2-(2,6-difluorophenyl)-N-(2,6-dimethylphenyl)-5-methylimidazo[1,2-a]pyridin-3-amine | C22 H19 F2 N3 | 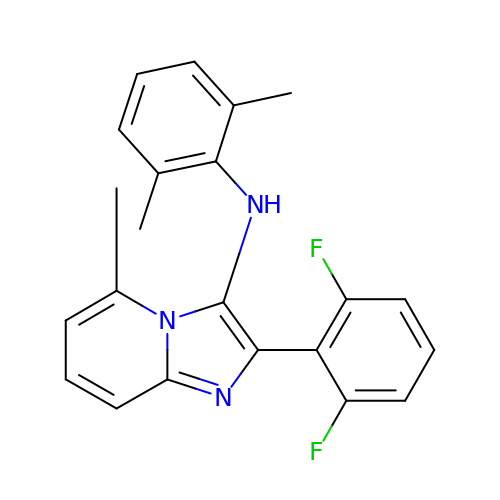RBMQZHVGMQCJOU-UHFFFAOYSA-N> GPGSIPDYQEQDIFLWRKETGFGFRILGGNEPGEPIYIGHIVPLGAADTDGRLRSGDELICVDGTPVIGKSH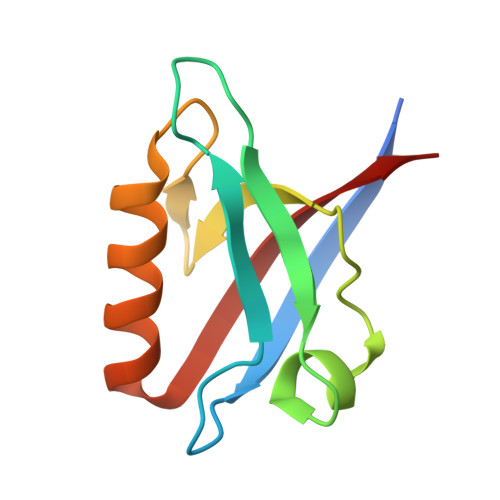QLVVQLMQQAAKQGHVNLTVRRKVV DIMETHYLFORMAMIDE | C3 H7 N 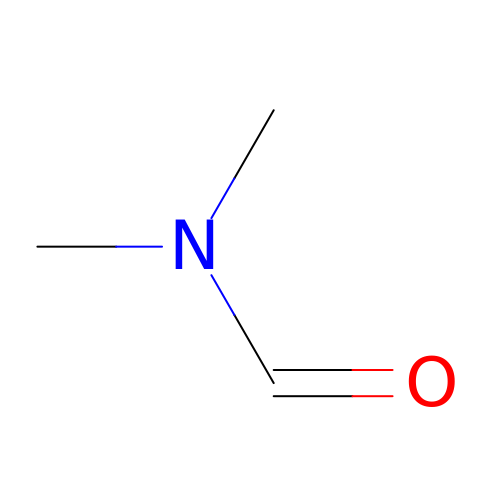O | ZMXDDKWLCZADIW-UHFFFAOYSA-N> MTVVGAVLPELKLYGDPTFIVSTALATRDFQDVHHDRDKAVAQGSKDIFVNILTDTGLVQRYVTDWAGPSALIKSIGLRLGVPWYAYDTVTFSGEVTAVNDGLITVKVVGRNTLGDHVTA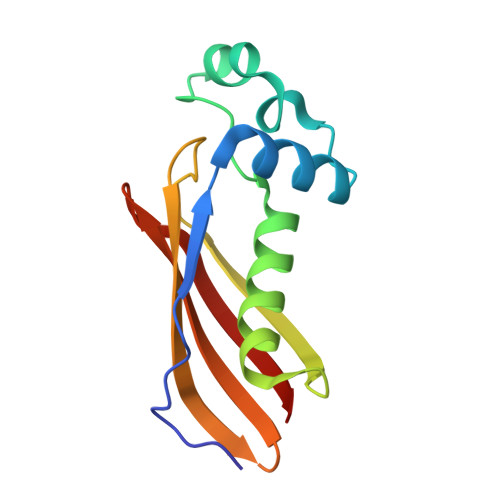TVELSMR> GSTVAAAVAAAGITGAAGTIPKQVYLRKRQQLFQLGGRGSEPGSFTWPRGLAVGPDNSI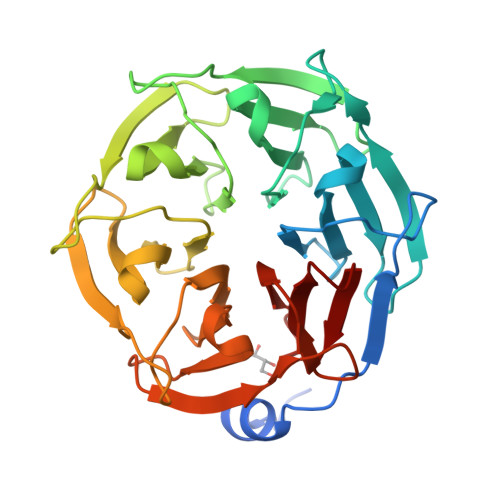VVADSSNHRVQVFDSNGIFVKEFGEYGNGEGEFDCLAGVAVNRIGQYIIADRYNHRIQVLDPQGRFLRAFGSQGTADGKFNYPWGVTTDALGFIYVCDKENHRVQVFQSDGSFVGKFGSCGRGEGQLEHPHYIAVSNTNRVIVSDSNNHRIQIFDVNGKVLSTVGGEGSDDGQFKFPRGVAVDDQGYIFVADSGNNRIQIFNPDGSFLKTFGSWGSGDSEFKGLEGVAIMSNGNILVCDRENHRVQVF>HHHHHHSSGLVPRGSAAEVGSGDNWHPGEELTQRSTQSHMFDGIS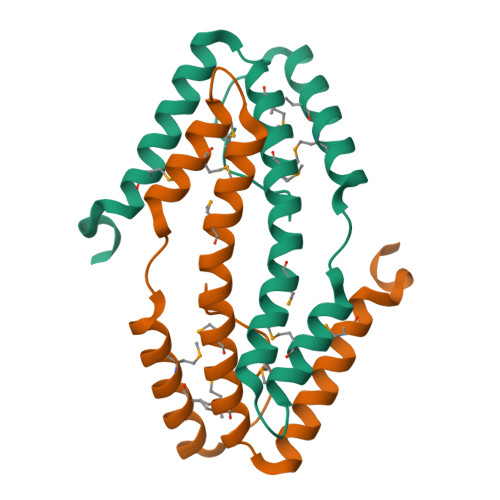LTEHQRQQMRDLMQQARHEQPPVNVSELETMHRLVTAENFDENAVRAQAEKMANEQIARQVEMAKVRNQMYRLLTPEQQAVLNEKHQQRMEQLRDVTQWQ[2x]> MAQKPRTVICVGDIHGYISKLNNLWLNLQSAIDPSDFSSALVIFLGDYCDRGPETRKVIDFLISLPEKHPDQTHVFLAGNHDFAFSGFLGLLPRPSDGSDLKDTWKEYSKSEETEGWYTGEGFEDMHLQGRRWAGKIKATFNSVKGMAYKGSIYDAGSTFESYGVPHGSSDLMKAVPESHKKFLTNMVWVHEEDDVCIETEEGLKHCKLIAVHAGLEKGNNVEEQLKLLRAKDTSISKIQHLSG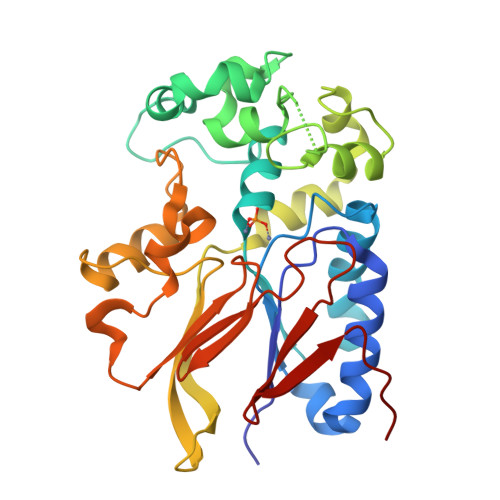RKNVWDIPQELDDKHTVVVSGHHGKLHIDGMRLIIDEGGGFPDKPVAAIVLPSKKIIRDTDNLSS>[2x]GMHSALQLRSRIKSSGELELSLDSIDTPHPGPDEVLIRIEASPLNPSDLGLLFGAADM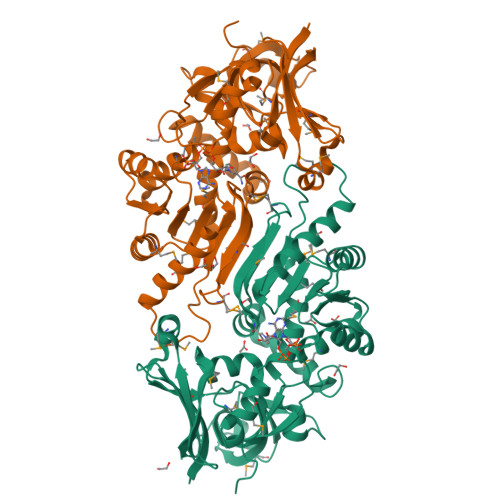STAKASGTAERPIVTARVPEGAMRSMAGRLDASMPVGNEGAGVVVEAGSSPAAQALMGKTVAAIGGAMYSQYRCIPADQCLVLPEGATPADGASSFVNPLTALGMVETMRLEGHSALVHTAAASNLGQMLNQICLKDGIKLVNIVRKQEQADLLKAQGAVHVCNAASPTFMQDLTEALVSTGATIAFDATGGGKLGGQILTCMEAALNKSAREYSRYGSTTHKQVYLYGGLDTSPTEFNRNFGMAWGMGGWLLFPFLQKIGRERANALKQRVVAELKTTFASHYSKEISLAEVLDLDMIAVYNKRATGEKYLINPNKGLAG> MAFPELLDRVGGRGRFQLLQAVALVTPILWVT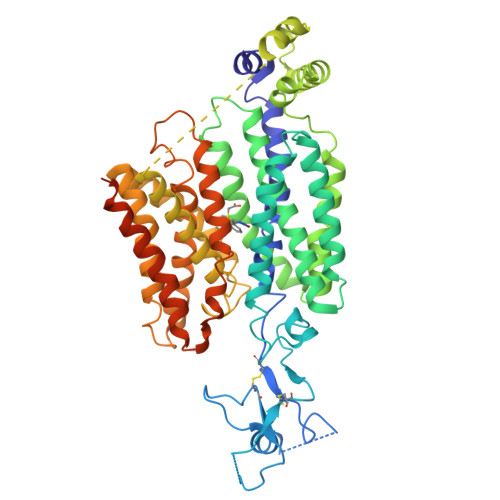TQSMLENFSAAVPHHRCWVPLLDNSTSQASIPGDFGRDVLLAVSIPPGPDQRPHQCLRFRQPQWQLIESNTTATNWSDADTEPCEDGWVYDHSTFRSTIVTTWDLVCDSQALRPMAQSIFLAGILVGAAVCGHASDRFGRRRVLTWSYLLVSVSGTIAALMPTFPLYCLFRFLVASAVAGVMMNTASLLMEWTSAQAGPLMMTLNALGFSFGQVLTGSVAYGVRSWRMLQLAVSAPFFLFFVYSWWLPESARWLITVGRLDQSLRELQRVAAVNRRKAEADTLTVEVLRSAMQEEPNGNQAGARLGTLLHTPGLRLRTFISMLCWFAFGFTFFGLALDLQALGSNIFLLQALIGIVDLPVKMGSLLLLSRLGRRLCQASSLVLPGLCILANILVPREMGILRSSLAVLGLGSLGAAFTCVTIFSSELFPTVIRMTAVGLGQVAARGGAMLGPLVRLLGVYGSWLPLLVYGVVPVLSGLAALLLPETKNLPLPDTIQDIQKQSVKKVTHDIAGGSVLKSARL>CGCNAAUUAGCG[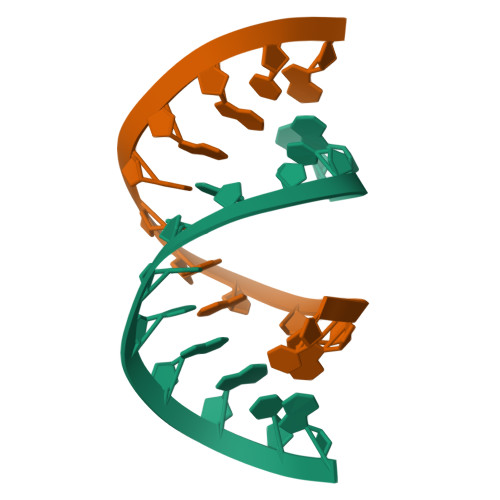2x]The human mitochondrial AAA+ protein LONP1 is a critical quality control protease involved in regulating diverse aspects of mitochondrial biology including proteostasis, electron transport chain activity, and mitochondrial transcription. The LONP1 protease consists of an N-terminal domain involved in substrate recognition and oligomerization, a AAA+ (ATPases associated with diverse cellular activities) domain that powers substrate translocation, and a C-terminal serine protease domain involved in substrate proteolysis. In mammals, LONP1 is a primary quality control protease responsible for regulating proteostasis and various biological functions within the mitochondrial matrix through diverse mechanisms. Here, we determine structures for human LONP1 in three different states: substrate-free, substrate-bound, and both substrate- and bortezomib-bound.

To test this prediction and characterize associated allosteric rearrangements, we determined a cryo-EM structure of substrate-bound human LONP1 incubated with saturating amounts of ATPγS and a 10-fold molar excess of bortezomib. Density for the bortezomib molecules was clearly visible in each of the six active sites, covalently attached to the catalytic serine and positioned within the substrate-binding groove, mimicking a proteolytic substrate. As predicted, bortezomib association with the protease active sites led to their reorganization to the active form previously observed for bacterial Lon. Importantly, the protease domains in LONP1Bz switch from the asymmetric conformation observed in our substrate-bound LONP1 structures to adopt a sixfold symmetric organization. This suggests that the presence of substrate in the protease active site induces rearrangement of the serine-containing catalytic loop, such that it extends toward the neighboring protease domain to allow formation of the proteolytically active S855-K898 catalytic dyad. Despite small differences in the spiraling ATPase conformations of substrate-bound human LONP1 and LONP1Bz, both structures show a similar engagement of a 12-residue translocating peptide by pore loop 1 aromatics. Intriguingly, we were unable to determine the interactions between pore loop 2 aromatics and substrate in our LONP1Bz structure, as these loops were not as well-ordered as they were in the substrate-bound LONP1 structure, suggesting a dissociation of substrate from these pore loop 2 residues prior to or after substrate association with the protease domain. Although our structure of LONP1Bz had bortezomib molecules bound to each of the subunits, thereby symmetrizing the protease domain, it is possible that all six protease active sites of human LONP1 are rarely, if ever, simultaneously activated for proteolytic activity.

>KDAIEEKFRERLKELVVPKHVMDVVDEELSKLGLLDNHSSEFNVTRNYLDWLTSIPWGKYSNENLDLARAQAVLEEDHYGMEDVKKRILEFIAVSQLRGSTQGKILCFYGPPGVGKTSIARSIARALNREYFRFSVGGMTDVAEIKGHRRTYVGAMPGKIIQCLKKTKTENPLILIDEVDKIGRGYQGDPSSALLELLDPEQNANFLDHYLDVPVDLSKVLFICTANVTDTIPEPLRDRMEMINVSGYVAQEKLAIAERYLVPQARALCGLDESKAKLSSDVLTLLIKQYCRESGVRNLQKQVEKVLRKSAYKIVSGEAESVEVTPENLQDFVGKPVFTVERMYDVTPPGVVMGLAWTAMGGSTLFVETSLRRPQDKDAKGDKDGSLEVTGQLGEVMKESARIAYTFARAFLMQHAPANDYLVTSHIHLHVPEGATPKDGPSAGCTIVTALLSLAMGRPVRQNLAMTGEVSLTGKILPVGGIKEKTIAAKRAGVTCIVLPAENKKDFYDLAAFITEGLEVHFVEHYREIFDIAF[6x]2-AMINOMETHYL-PYRIDINE | C6 H8 N2 | 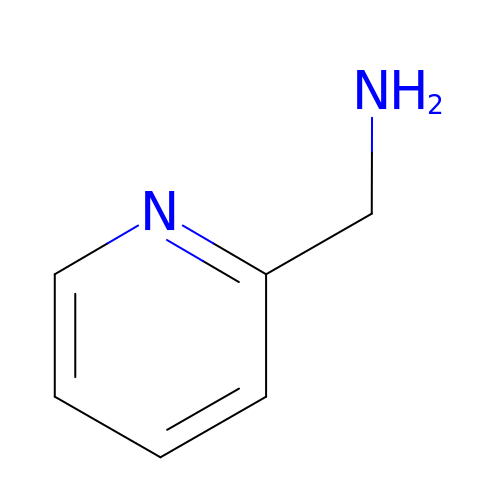WOXFMYVTSLAQMO-UHFFFAOYSA-N3-[(piperidin-1-yl)methyl]benzoic 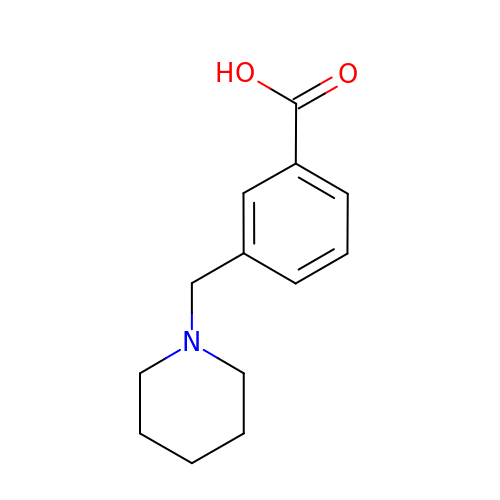acid | C13 H17 N O2 | UIXWGRXBYZGOQK-UHFFFAOYSA-N> DPSNVETYEQILQWVTEVLGNDIPHDLIIGTADIFIRQLKENEENEDGNIEERKEKIQHELGINIDSLKFNELVKLMKNINKRALPNIENDIIKLSDSKTSNIESVPIYSIDEFFLQRKLRSELGYKDTSVIQDLSEKILNDIETLEHNPVALEQKLVDLLKFENISLAEFILKNRSTIFWGIRLAKSTENEIPNLIEKMVAKGLNDLVEQYKFRENPAIPPVIDLEKIKFDESSKLMTVTKVSLPEGSFKRVKPQYDEIHIPAPSKPVIDYELKEITSLPDWCQEAFPSSETTSLNPIQSKVFHAAFEGDSNMLICAPTGSGKTNIALLTVLKALSHHYNPKTKKLNLSAFKIVYIAPLKALVQEQVREFQRRLAFLGIKVAELTGDSRLSRKQIDETQVLVSTPEKWDITTRNSNNLAIVELVRLLIIDEIHLLHDDRGPVLESIVARTFWASKYGQEYPRIIGLSATLPNYEDVGRFLRVPKEGLFYFDSSFRPCPLSQQFCGIKERNSLKKLKAMNDACYEKVLESINEGNQIIVFVHSRKETSRTATWLKNKFAEENITHKLTKNDAGSKQILKTEAANVLDPSLRKLIESGIGTHHAGLTRSDRSLSEDLFADGLLQVLVCTATLAWGVNLPAHTVIIKGTDVYSPEKGSWEQLSPQDVLQMLGRAGRPRYDTFGEGIIITDQSNVQYYLSVLNQQLPIESQFVSKLVDNLNAEVVAGNIKCRNDAVNWLAYTYLYVRMLASPMLYKVPDISSDGQLKKFRESLVHSALCILKEQELVLYDAENDVIEATDLGNIASSFYINHASMDVYNRELDEHTTQIDLFRIFSMSEEFKYVSVRYEEKRELKQLLEKAPIPIREDIDDPLAKVNVLLQSYFSQLKFEGFALNSDIVFIHQNAGRLLRAMFEICLKRGWGHPTRMLLNLCKSATTKMWPTNCPLRQFKTCPVEVIKRLEASTVPWGDYLQLETPAEVGRAIRSEKYGKQVYDLLKRFPKMSVTCNAQPITRSVMRFNIEIIADWIWDMNVHGSLEPFLLMLEDTDGDSILYYDVLFITPDIVGHEFTLSFTYELKQHNQNNLPPNFFLTLISENWWHSEFEIPVSFNGFKLPKKFPPPTPLLENISISTSELGNDDFS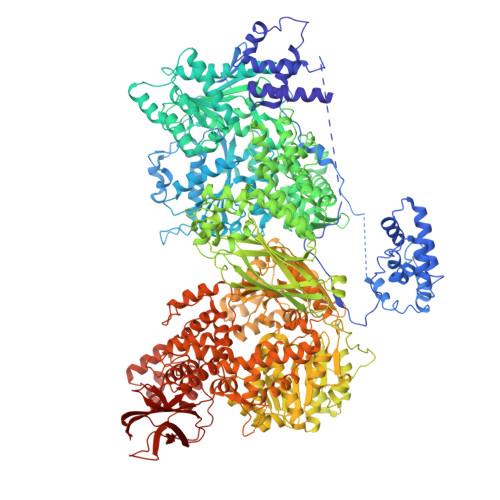EVFEFKTFNKIQSQVFESLYNSNDSVFVGSGKGTGKTAMAELALLNHWRQNKGRAVYINPSGEKIDFLLSDWNKRFSHLAGGKIINKLGNDPSLNLKLLAKSHVLLATPVQFELLSRRWRQRKNIQSLELMIYDDAHEISQGVYGAVYETLISRMIFIATQLEKKIRFVCLSNCLANARDFGEWAGMTKSNIYNFSPSERIEPLEINIQSFKDVEHISFNFSMLQMAFEASAAAAGNRNSSSVFLPSRKDCMEVASAFMKFSKAIEWDMLNVEEEQIVPYIEKLTDGHLRAPLKHGVGILYKGMASNDERIVKRLYEYGAVSVLLISKDCSAFACKTDEVIILGTNLYDGAEHKYMPYTINELLEMVGLASGNDSMAGKVLILTSHNMKAYYKKFLIEPLPTESYLQYIIHDTLNNEIANSIIQSKQDCVDWFTYSYFYRRIHVNPSYYGVRDTSPHGISVFLSNLVETCLNDLVESSFIEIDDTEAETEIISTLSNGLIASHYGVSFFTIQSFVSSLSNTSTLKNMLYVLSTAVEFESVPLRKGDRALLVKLSKRLPLRFPEHTSSGSVSFKVFLLLQAYFSRLELPVDFQNDLKDILEKVVPLINVVVDILSANGYLNATTAMDLAQMLIQGVWDVDNPLRQIPHFNNKILEKCKEINVETVYDIMALEDEERDEILTLTDSQLAQVAAFVNNYPNVELTYSLNNSDSLISGVKQKITIQLTRDVEPENLQVTSEKYPFDKLESWWLVLGEVSKKELYAIKKVTLNKETQQYELEFDTPTSGKHNLTIWCVCDSYLDADKELSFEINVK> SAMNNEGKALMAIKGSFSNLVNMLLDWDDVHNSDLCSWRGVFCDNVSYSVVSLNLSSLNLGGEISPAIGDLRNLQSIDLQGNKLAGQIPDEIGNCASLVYLDLSENLLYGDIPFSISKLKQLETLNLKNNQLTGPVPATLTQIPNLKRLDLAGNHLTGEISRLLYWNEVLQYLGLRGNMLTGTLSSDMCQLTGLWYFDVRGNNLTGTIPESIGNCTSFQILDISYNQITGEIPYNIGFLQVATLSLQGNRLTGRIPEVIGLMQALAVLDLSDNELVGPIPPILGNLSFTGKLYLHGNMLTGPIPSELGNMSRLSYLQLNDNKLVGTIPPELG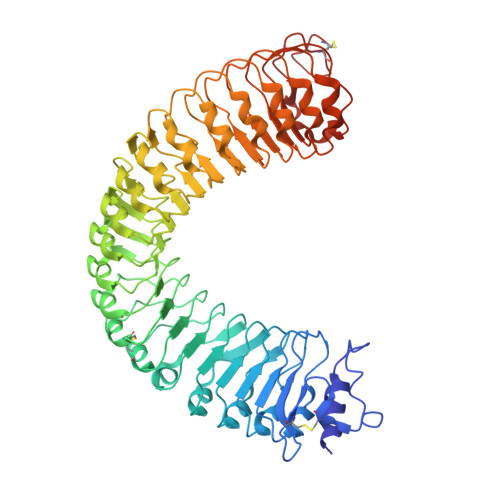KLEQLFELNLANNRLVGPIPSNISSCAALNQFNVHGNLLSGSIPLAFRNLGSLTYLNLSSNNFKGKIPVELGHIINLDKLDLSGNNFSGSIPLTLGDLEHLLILNLSRNHLSGQLPAEFGNLRSIQMIDVSFNLLSGVIPTELGQLQNLNSLILNNNKLHGKIPDQLTNCFTLVNLNVSFNNLSGIVPPMKNFSRFAPASFVGNPYLCGNWVGSICGPHHHHHH>MTRNQLHNWLNAGFFGLLLLLIHVQGQDSPEANPIRNTHTGQIQGSLIHVKDTKAGVHTFLGIPFAKPPVGPLRFAPPEAPEPWSGVRDGTAHPAMCLQNLDMLNEAGLPDMKMMLSSFPMSEDCLYLNIYTPAHAHEGSNLPVMVWIHGGALVIGMASMFDGSLLTVNEDLVVVTIQYRLGVLGFFSTGDQHARGNWGYLDQAAALRWVQQNIAHFGGNPDRVTIFGESAGGTSVSSHVVSPMSQGLFHGAIMESGVALLPDLISETSEMVSTTVAKLSGCEAMDSQALVRCLRGKSEAEILAINKVFKMIPAVVDGEFFPRHPKELLASEDFHPVPSIIGVNNDEFGWSIPVVMGSAQMIKGITRENLQAVLKDTAVQMMLPPECSDLLMEEYMGDTEDAQTLQIQFTEMMGDFMFVIPALQVAHFQRSHAPVYFYEFQHPPSYFKDVRPPHVKADHADEIPFVFASFFWGMKLDFTEEEELLSRRMMKYWANFARHGNPNSEGLPYWPVMDHDEQYLQLDIQPAVGRALKAGRLQFWTKTLPQKIQELKAS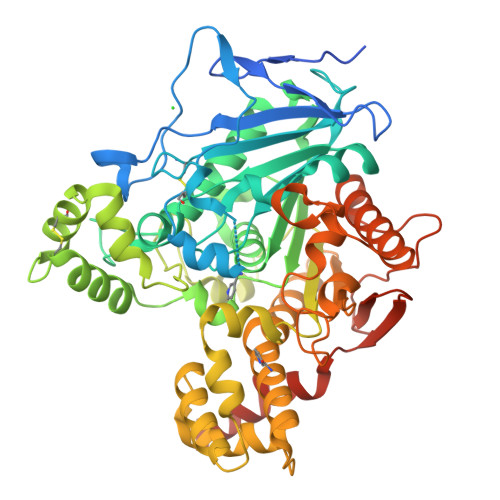QDKHREL[4x]>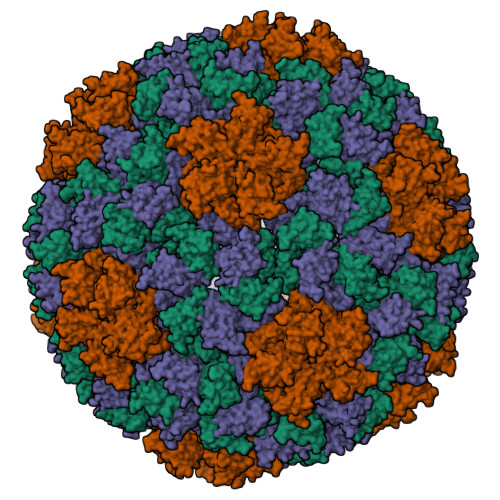[3x]PVTLEPMPPGEGAQEGEPPTVEARYKSFSIKMLKDMKEGVKQYGPNSPYMRTLLDSIAHGHRLIPYDWEILAKSSLSPSQFLQFKTWWIDGVQEQVRRNRAANPPVNIDADQLLGIGQNWSTISQQALMQNEAIEQVRAICLRAWEKIQDPGSACPSFNTVRQGSKEPYPDFVARLQDVAQKSIADEKARKVIVELMAYENANPECQSAIKPLKGKVPAGSDVISEYVKACDGIGGAMHKAMLMAQLE>MNQNLLVTKRDGSTERINLDKIHRVLDWAAEGLHNVSISQVELRSHIQFYDGIKTSDIHETIIKAAADLISRDAPDYQYLAARLAIFHLRKKAYGQFEPPALYDHVVKMVEMGKYDNHLLEDYTEEEFKQMDTFIDHDRDMTFSYAAVKQLEGKYLVQNRVTGEIYESAQFLYILVAACLFSNYPRETRLQYVKRFYDAVSTFKISLPTPIMSGVRTPTRQFSSCVLIECGDSLDSINATSSAIVKYVSQRAGIGINAGRIRALGSPIRGGEAFH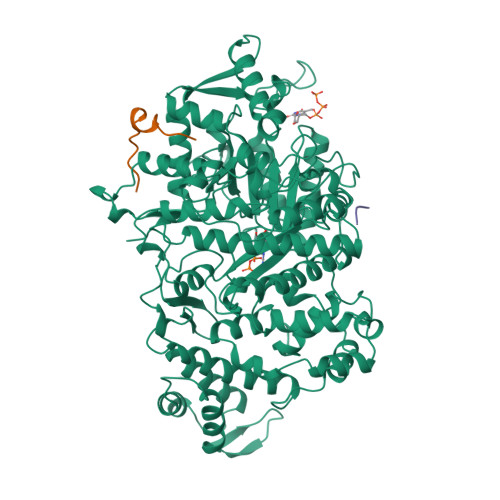TGCIPFYKHFQTAVKSASQGGVRGGAATLFYPMWHLEVESLLVLKNNRGVEGNRVRHMDYGVQINKLMYTRLLKGEDITLFSPSDVPGLYDAFFADQEEFERLYTKYEKDDSIRKQRVKAVELFSLMMQERASTGRIYIQNVDHCNTHSPFDPAIAPVRQSNLCLEIALPTKPLNDVNDENGEIALCTLSAFNLGAINNLDELEELAILAVRALDALLDYQDYPIPAAKRGAMGRRTLGIGVINFAYYLAKHGKRYSDGSANNLTHKTFEAIQYYLLKASNELAKEQGACPWFNETTYAKGILPIDTYKKDLDTIANEPLHYDWEALRESIKTHGLRNSTLSALMPSETSSQISNATNGIEPPRGYVSIKASKDGILRQVVPDYEHLHDAYELLWEMPGNDGYLQLVGIMQKFIDQSISANTNYDPSRFPSGKVPMQQLLKDLLTAYKFGVKTLYYQNTRDGAEDAQDDLVPSIQDDGCESGACKI[3x];>[4x]YLVGQIDSEVDTDDLSNFQL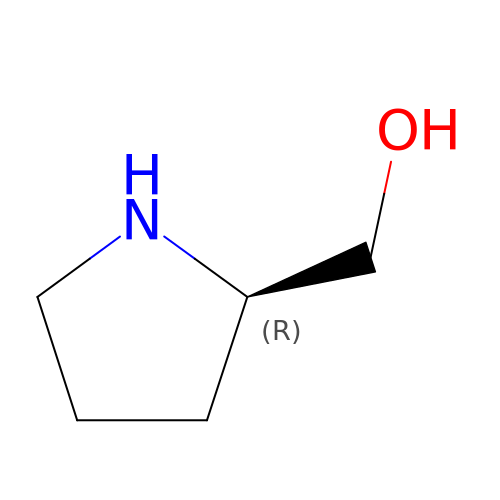D-Prolinol | C5 H11 N O | HVVNJUAVDAZWCB-RXMQYKEDSA-N>GSHMTAPTVPVALVTGAAKRLGRSIAEGLHAEGYAVCLHYHRSAAEANALSATLNARRPNSAITVQADLSNVATAPVSGADGSAPV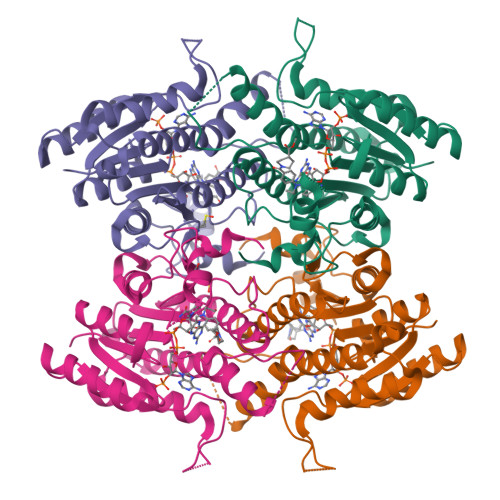TLFTRCAELVAACYTHWGRCDVLVNNASSFYPTPLLRNDEDGHEPCVGDREAMETATADLFGSNAIAPYFLIKAFAHRVAGTPAKHRGTNYSIINMVDAMTNQPLLGYTIYTMAKGALEGLTRSAALELAPLQIRVNGVGPGLSVLVDDMPPAVWEGHRSKVPLYQRDSSAAEVSDVVIFLCSSKAKYITGTCVKVDGGYSLTRA[4x]>MSSTVIAFGDPKAQKKWSSELAVDIRKKSYFESRFIGTSENAVIQRKTEVESDAGDRVSFDLSVRLRGQPTFGDDRVEGKEENLKFYTDEVIIDQVRHSVSAGGRMSRKRTAHDLRKTGRDRLGDYFYQLTDELFFMYLSGARGINKDFILPTSFTGYAKNPFNTPDAAHLLYGGVATSKASLANTDTMSRVVIERANVQATMMQAQDPETANMVPVSVEGEDRYVCVMSPFQEHSLRTSDAAGWLEIQKAAAAAEGRNNPIFKGGLGMIGNTVLHSHRNVVRFSDYGAGSDQPAARALFMGRQAAVVAYGTKGGLRYDWQEETKDYGNEPTVASGFIAGIKKTRFNDRDFGVISIDTYAKDPNPNNPA[9x];>[9x]MALIQSDFAQGIRMTPVPDCAG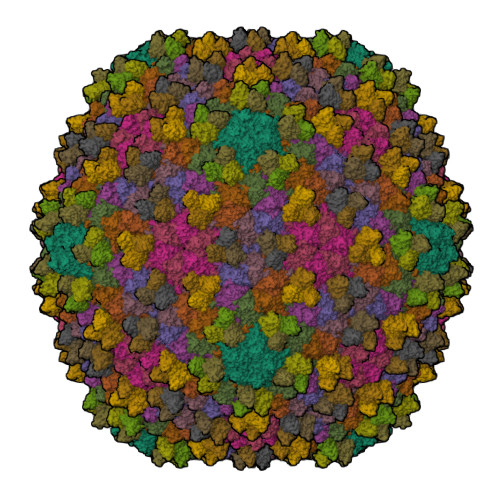DVTACRFDITLKNAPAAGDIIELGVLPGNAVPVEAILDVDDLDTGGAPTITLDVGIMSGPVGKNDPARTCGNELFAASTVGQAGGVVRATASSAFRIQKAEDHRSVGVKVAAGPATGAAGKTIALILFYVQGTSQ2-METHYLBUTANOIC ACID | C5 H10 O2 | 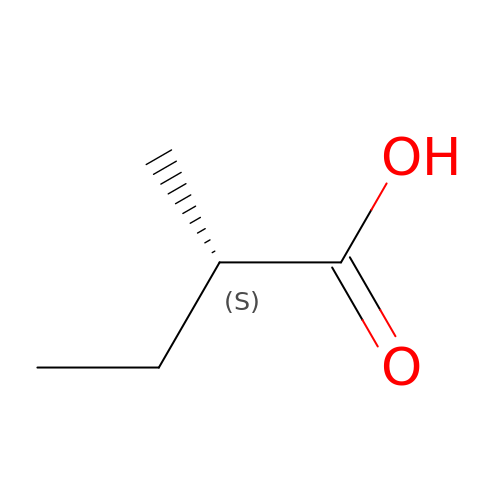WLAMNBDJUVNPJU-BYPYZUCNSA-N> MGHHHHHHHHHHSSGHIDDDKHMVNVKKEFVDNMFSVKGKVALVTGATGALGCVLSKAYGYAG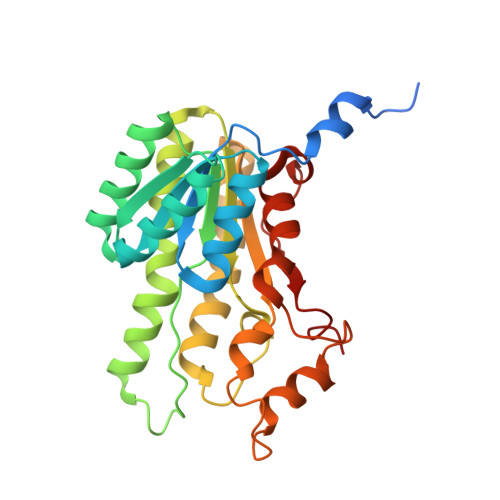AKVFMTGRNEKKLQALEAEFKAEGIDCAYGVADPADEAQVDAMITACVAQYGEVNILAVTHGFNKPQNILEQSVADWQYIMDADCKSVYVVCKYVAQQMVDQGKGGKIVVVTSQRSKRGMAGYTGYCTSKGGADLMVSSMACDLSAKYGINVNSICPTVFRSDLTEWMFDPESAVYQNFLKREPIGRLAEPEDFVGYALFLSSDASNYITGANCDCSGGYLTC> MGHHHHHHMLHLLEQIRAYCETCWEWQEAHEPGMDQDKNPMPAPVEHQICPAVCVLMKLSFDEEHRHAMNELGGLQAIAELLQVDCEMYGLTNDHYSITLRRYAGMALTNLTFGDVANKATLCSMKGCMRALVAQLKSESEDLQQVIASVLRNLSWRADVNSKKTLREVGSVKALMECALEVKKESTLKSVLSALWNLSAHCTENKADICAVDGALAFLVGTLTYRSQTNTLAIIESGGGILRNVSSLIATNEDHRQILRENNCLQTLLQHLKSHSLTIVSNACGTLWNLSARNPKDQEALWDMGAVSMLKNLIHSKHKMIAMGSAAALRNL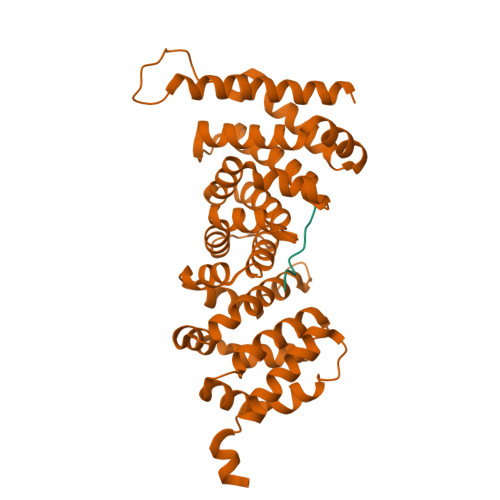MANRPAKYKDANIMSPGSSLPS;> YQGGGEEMALP> QSLQVKPLQVEPPEPVVAVALGASRQLTCRLACADRGASVQWRGLDTSLGAVQSDTGRSVLTVRNASLSAAGTRVCVGSCGGRTFQHTVQLLVYAFPNQLTVSPAALVPGDPEVACTAHKVTPVDPNALSFSLLVGGQELEGAQALGPEVQEEEEEPQGDEDVLFRVTERWRLPPLG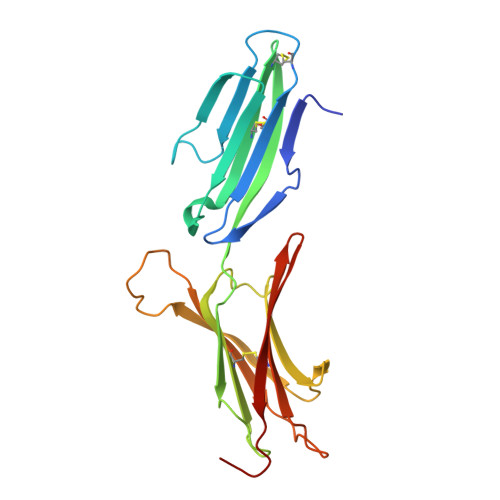TPVPPALYCQATMRLPGLELSHRQAIPVLIEGR>MAHHHHHHMLKLIVETKTLVQSLGFASSVVEKRNVIPEYANIKLSAKDGNLELSSTNMDLYLSQKIAVQVVSEGECTVSTKTLNDIVRKLPDSELTLTDLGTTGLEIKGKNCKFNLFTLPVSSFPAMDSINPEASFKISCTDFAKIIESTKFSISLDETRYNLNGVYLHIKDKEFCSASTDGHRLSISWVTLEKQIKNFGVILPQKSAEEILKIVKDPKNINEDIEILLSSNKIKFICNENTSMLSKLIDGTFPDYSTFIPESSSSKLVINRKMFADSIERIAIITVEKFRAVKLSLSRETLEISAVGEARGNAKEVINSSQDKESFYEYNSDESLAIGFNPQYLEDVLKAVKSDVVELYFSDVSAPVLIKFPENPKDIFVVMPVKV[2x]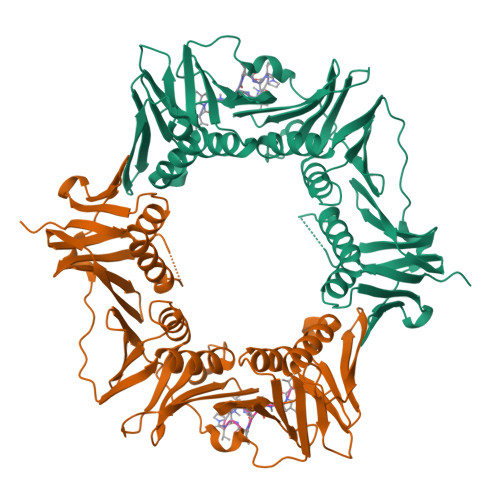;>XVPTLPLVPXG[2x]5-chloro-1H-indole-2-carboxylic 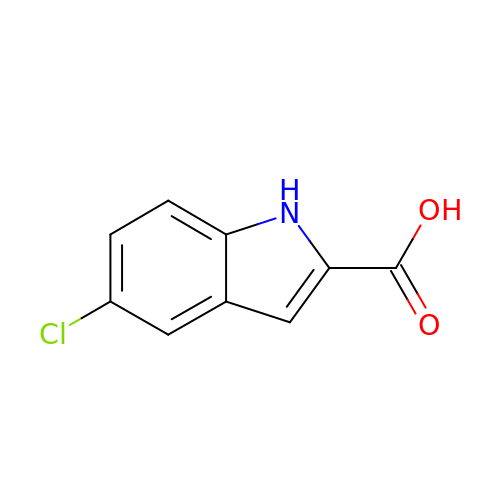acid | C9 H6 Cl N O2 | FUQOTYRCMBZFOL-UHFFFAOYSA-N>MAAEGYGAASPATATTQDGAKGAAPPNPAASINSPAPAANPEKLTPAQLKAKAKAEKQARRAAAKEAKSAVAAAGQPAQQSGSAGADSKGAAKGKGKQEGQQVPPKGVLVHRPSVSGRRPSIMVVEKDARSGIPECFSHIPMAKRIPTSQAHKDVHPAVLAVGQQMATFALKDSISRLKATLLAFRKVIESYETPKGNSLSRHFVPHVLNPQIEYLTECRPMCFAMGNAIRLLKAKVNKFDINTPEDEAKEGLLEWIDFLINERITLAEYVIARNAAQSINDGDTIVTYGRHRLVEKTLLRARKEGKSFNVTVLDDPYVGEGKELAKVLRHAGIPVLYSPNLGGLRSKVPAASNVFLGGEAIFANGSLHAPSGTADVAMAATNAGAKVIVLCETINFDRERVSVDALTYNEIDPERNTGDCFRLLFDNTHERYITGVITEIEFGGGNSPAQAILALLRKQEDPLIA[2x];>[2x]MAPSQASHTPSLATWTKSLRDQSLEASIESLIFLLKRRQVTGDECAGAIAQLLRQVVAKSKWHDVDQLLYRVQTAGARLARAAPHEPVIGNIVRRVLGLIRDEASENRNADDIASDAASDIQSLAPSQPPPQQRPPPPARTLTSGLQVSKSMFNLLSVADPSESPVTGASTPISQAQQPFSVHALRSEVMDGIEEILDEINQADDQIASFAEIQIHPGDYVLAYQ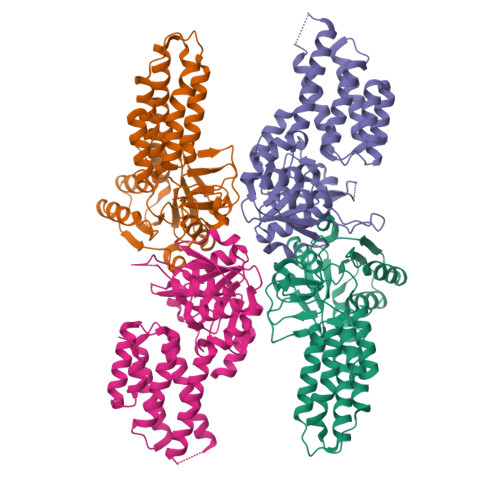PSKTVERFLVKAASKRRFTVILASLNPPAPGEEEQPYAALRKKLNAAGVSTINLASNGLMAYIPRVNKVIFGAKAVYQNGGLLVDSGACIAAQAAHEYLKPVIALCGVYKFCPEDPSDEVSRGELGNPSSYVSYADGPELDSFEVENTTTDYIPPDLVDVYLTNLGPQTRHHLGGIYADHYKIEDIGFSLQVGE> GSPPDPQVRCPSVIEFGKYEIHTWYSSPYPQEYSRLPKLYLCEFCLKYMKSRTILQQHMKKCGWFHPPANEIYRKNNISVFEVDGNVSTIYCQNLCLLAKLFLDHKTLYYDVEPFLFYVLTQNDVKGCHLVGYFSKEKHCQQKYNVSCIMILPQYQRKGYGRFLIDFSYLLSKREGQAGSPEKPLSDLGRLSYMAYWKSVILECLYHQNDKQISIKKLSKLTGICPQDITSTLHHLRMLDFRSDQFVIIRREKLIQDHMAKLQLNLRPVDVDPECLRWTPVIVSNS;> QTARKSTGGKAPRKQLATK

KAT6A and KAT6B are members of the MYST family of acetyltransferases, a group of transcriptional regulators implicated in cellular proliferation and development. The hallmark of this family, which includes KAT5, KAT6A, KAT6B, KAT7, and KAT8 (also known as Tip60, MOZ, MORF, HBO1, and MOF, respectively), is the MYST acetyltransferase domain (herein referred to as the MYST domain) that employs acetyl-CoA to catalyze acetylation of lysine residues within the histone tails of the nucleosome. KAT6A forms a 4-protein complex with BRPF1, ING4/5, and MEAF6 to acetylate H3K23. We show that the MYST domain and KAT6AFL preferentially acetylate H3K14, with this selectivity linked to a glycine pair preceding K14.

While our efforts to obtain crystallographic data for this complex were unsuccessful, we were able to solve a crystal structure of the MYST domain bound to a H3K14-CoA bisubstrate inhibitor. Such peptide-CoA conjugates have been utilized to interrogate the binding sites of acetyltransferases so we evaluated how H3K14-CoA, which consists of H3 (5-23) with the ε-amino group of K14 covalently attached to CoA through a non-native acetyl bridge, is bound to the KAT6A MYST domain. The structure of the KAT6A MYST domain with H3K14-CoA was solved at 1.72 Å resolution, with interpretable electron density observed for residues 10 to 17 of the H3 peptide, the CoA moiety, and the acetyl bridge between the H3K14 ε-amino group and CoA. Comparing this structure with prior crystallographic models of the KAT6A MYST domain bound to acetyl-CoA and NuA4 complexed with a Htz1 peptide indicates that the CoA and peptide portions of the H3K14-CoA bisubstrate inhibitor largely overlap with acetyl-CoA and the Htz1 peptide, respectively. This observation implies that the bisubstrate inhibitor occupies both the acetyl-CoA and peptide binding sites of the KAT6A MYST domain, as expected. The structure shows the peptide portion of the bisubstrate inhibitor surrounded by three loops within the MYST domain: α2-β7, β8-β9, and α3-α4. Within this crevice, the bound peptide assumes a β-turn, resembling a type I conformation based on dihedral angles (ϕ, ψ) of G13 (−90.1°, −6.9°) and K14 (−118.1°, 5.3°). In addition, we note that the α-carbon atoms G12 and G13 are in proximity (3.3–5.0 Å) to several residues within the α2-β7 (autoacetylated K604, L606, and F613), β8-β9 (E635, S645, and C646), and α3-α4 (E680) loops. Steric restrictions within this environment provide a model for the preferred acetylation of lysine residues adjacent to a GG pair given the small size and conformational flexibility of glycine. The peptide portion of the bisubstrate inhibitor is stabilized by several putative hydrogen bonds, including 8 water-mediated contacts and 8 direct contacts with the KAT6A MYST domain.>MGEPAKIYINLGVQAPGPFGGGTPEEVAATLDRVKAAAPGIGIIVDLDEGSGVHRDSDHVRLYPEGAGRYTLAEEQAIVDHAKALGAEICYHLNLTVFLPTDPVSEEERAAAKPVWTWTGLHHCIPKEKLLETLLPQKLDELEAAFPGKLDYVYLDRLFDGRCYDLTDEEVRYVLDLIKERGLGIKIESTKYLDTILESGVKVLVDEAVSEKNFDTGKAKVLD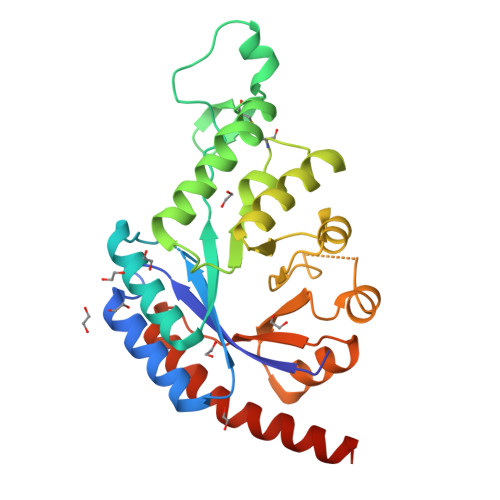PKLFEKYPDLITVEVLYESIETIERALAAGVRNIAIHFGGYGVVSQLDEILDGVRAITENILALASAGSGHHHHHH[2x]> ASPQVSVTLQLVVDSSMFAKYNGDAKKIVTVLDTRVNIMKSIFKPLLLLITLSGIEMWTSKDLIT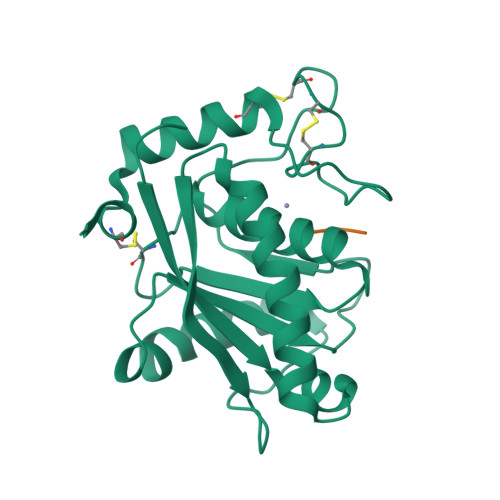VKPAGDLTLSLFADWRQTLLLSRILNDNAQLQTAVDFRGAVVGLAFVGTMCNAKYSAGIIQDFSAIPLLMAVVMAHELGHNLGMLHDDGYSCDCDVCIMAPSLSSDPTKVFSNCSLILYEDFLSNEEPDCIDNASNN;> KNL>GSAAFNAWRNTPKSLINLKEIEPQLATDPDSAFFWSGRTEGVGGPDVAEAIAKSRGGVTLESTIKDKNIKMPEWDFDNPQSIKAWEDVSASYAKQVSGEVRAVVGQSLREGNIWENVELPRLMGNDNVTKITTIDPLSQTEKVIFVRDN[2x]

Here, we identify and characterize a novel toxin domain in Pantoea ananatis that displays remarkable structural and functional conservation with the human enzyme CD38. This bacterial toxin, fused to a type VI secretion system (T6SS) PAAR domain, harbors a C-terminal ADP-ribosyl cyclase (ARC) domain that hydrolyzes NAD+ and NADP+in vitro and in vivo, leading to growth inhibition in both bacterial and eukaryotic cells. We show that this bacterial toxin, designated ARCtox, shares the catalytic residues, enzymatic activity, and overall fold of CD38, yet functions as a cytotoxic effector capable of depleting NAD+ and NADP+ in both bacteria and eukaryotic target cells, suggesting a dual role in microbial competition and host interaction. We demonstrate that the C-terminal extension of a specialized PAAR protein from P. ananatis, PANA_2924, acts as a potent cytotoxic effector, exhibiting both antibacterial and anti-eukaryotic activity through depletion of the cellular NAD+/NADP+ pool.

Crystallization of the PANA_2924 extension was, however, achieved after dissociating the immunity protein from the complex by adding urea to the affinity chromatography washing buffer, followed by refolding and SEC purification of the isolated toxin. An X-ray diffraction dataset was collected, and the structure was solved by molecular replacement using the AlphaFold3 model, followed by refinement to a resolution of 1.6 Å. PANA_2924 crystallized in the space group P212121, with two molecules per asymmetric unit. These two molecules adopt similar conformations. However, while the first chain could be modeled from residues 252 to 385, missing a flexible loop from 311 to 317, the second chain could be modeled from residues 250 to 385, missing a different flexible loop (amino acids 345–349). The structure reveals a globular fold with two lobes, consisting of a four-stranded β-sheet covered by a helical cap composed of five α-helices. A search for structural homologues using DALI showed that the PANA_2924 C-terminal extension displays a fold similar to the human protein CD38 (Z-score: 8.6). Although the overall identity of the PANA_2924-C and CD38 domains retrieved using DALI is relatively low (26.3%), the two domains are indeed structurally similar. Indeed, substitution of any of the ARCtox putative catalytic residues, W273, E299, W323, and E356, by alanines abolished ARCtox activity in E. coli. Upon incubation with ARCtox, NAD+ and NADP+ were converted into nicotinamide and ADP-ribose.>GSMATEEHQRLASIVKSCHESLRQLTKEYGATAAWQEHTSPRNAKQLAEYAKAMKQLAAIWETNDGKVELQARSRIKWAIDYITKYFFTEGIYLQKRQREQRLLESYRAEGKLGEVQCRLMEEPPDRLHVLDVGSCFNPFSSAPHLEVTALDLCPATEDVLQADFLKVEVVPGIREPELEEGSVRRLPASHYECVIFSLLLEYMPSAEQRLQCCLQAYDLLLPEGILVLITPDSQHVGKNAHLMKNWRYSLARIGLLRVRFEKLPHISCMVF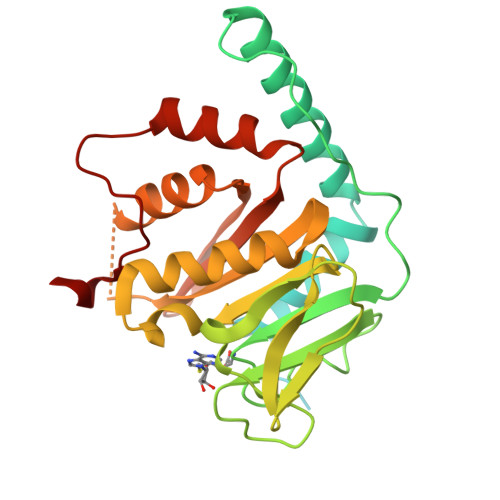RKAISRELSQHWASIHREEGMCEEIRIPQDDS[4x]> MDVASSDTVYTFPDEFKLGAATASYQIEGAWDENGKGPNIWDTLTHEHPDYVVDGATGDIADDSYHLYKEDVKILKELGAQVYRFSISWARVLPEGHDNIVNQDGIDYYNNLINELLANGIEPMVTMYHWDLPQALQDLGGWPNL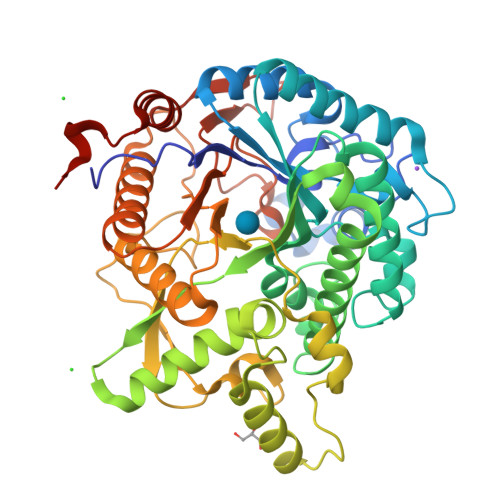VLAKYSENYARVLFKNFGDRVKLWLTFNAPLTFMDGYASEIGMAPSINTPGIGDYLAAHTVIHAHARIYHLYDQEFRAEQGGKVGISLNINWCEPATNSAEDRASCENYQQFNLGLYAHPIFTEEGDYPAVLKDRVSRNSADEGYTDSRLPQFTAEEVEYIRGTHDFLGINFYTALLGKSGVEGYEPSRYRDSGVILTQDAAWPISASSWLKVVPWGFRKELNWIKNEYNNPPVFITENGFSDYGGLNDTGRVHYYTEHLKEMLKAIHEDGVNVIGYTAWSLMDNFEWLRGYSEKFGIYAVDFEDPARPRIPKESAKVLAEIMNTRKIPERFRDLEHHHHHH> MSVLNTPNHYKMDNSGRRVVIDPVTRIEGHMRCEVNVDENNVIQNAVSTGTMWRGLEVILRGRDPRDAWAFVERICGVCTGCHALASVRAVEDALDIKIPHNATLIREIMAKTLQIHDHIVHFYHLHALDWVNPVNALKADPQATSELQKLVSPHHPMSSPGYFKDIQIRIQKFVDSGQLGIFKNGYWSNPAYKLSPEADLMAVTHYLEALDFQKEIVKIHAIFGGKNPHPNYMVGGVPCAINIDGDMAAGAPINMERLNFVKSLIEQGRTFNTNVYVPDVIAIAAFY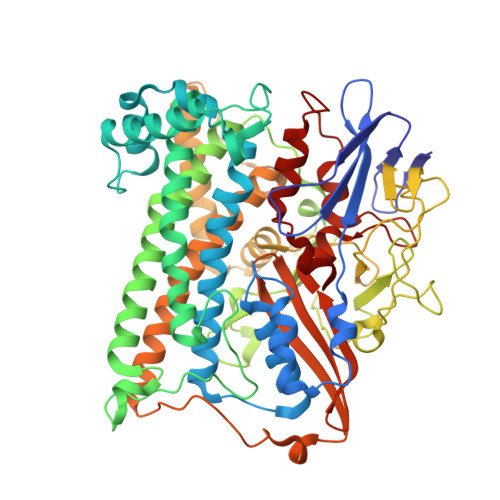RDWLYGGGLSATNVMDYGAYPKTPYDKSTDQLPGGAIINGDWGKIHPVDPRDPEQVQEFVTHSWYKYPDETKGLHPWDGITEPNYELGSKTKGSRTNIIEIDESAKYSWIKSPRWRGHAVEVGPLARYILAYAQGVEYVKTQVHTSLNRFNAVCRLLDPNHKDITDLKAFLGSTIGRTLARALESEYCGDMMLDDFNQLISNIKNGDSSTANTDKWDPSSWPEHAKGVGTVAAPRGALAHWIVIEKGKIKNYQCVVPTTWNGSPRDPKGNIGAFEASLMGTPMERPDEPVEVLRTLHSFDPCLACSTH>MKFTYLVSLAAFAVTALGSRPTPPNLEFLFSANLTKGPAYIYDQSDAQIKALQTLTGGIIAGPNFDGTVIGGTALSTRGADGTIRADAHYLIQTSDGANILVTESAAI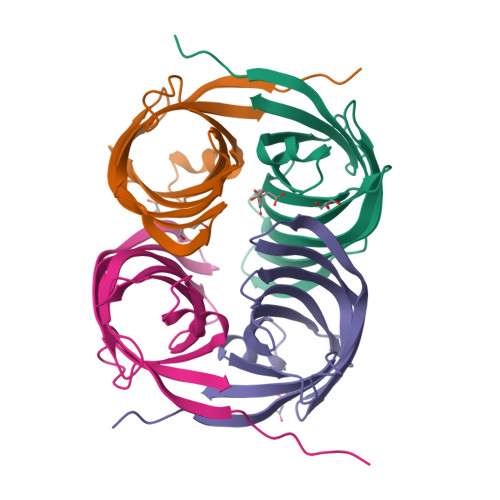PYVAVLFDTSSEKYNWLNNVTAWGTPPNLNEINFLEYWQIE[4x]> GSPSRAEYRNWSKPQCNITGFAPFSKDNSIRLSAGGDIWVTREPYVSCDPDKCYQFALGQGTTLNNGHSNDTVHDRTPYRTLLMNELGVPFHLGTKQVCIAWSSSSCHDGKAWLHVCVTGDDENATASFIYNGRLVDSIGSWSKKILRTQESECVCINGTCTVVMTDGSASGKADTKILFIEEGKIVHTSPLSGSAQHVEECSCYPRYPGVRCVCRDNWKGSNRPIVDINVKDYSIVSSYVCSGLVGDTPRKNDSSSSSHCLDPNNEEGGHGVKGWAFDDGNDVWMGRTISE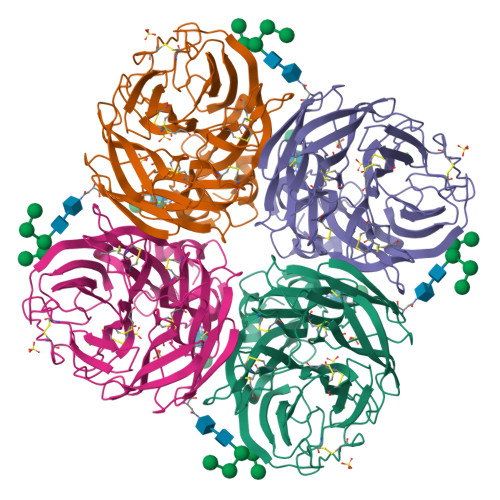KLRSGYETFKVIEGWSKPNSKLQINRQVIVDRGNRSGYSGIFSVEGKSCINRCFYVELIRGRKQETEVLWTSNSIVVFCGTSGTYGTGSWPDGADINLMPI(2~{R})-2-[5-[3-chloranyl-2-methyl-5-(4-methylpiperazin-1-yl)-4-oxidanyl-phenyl]-6-ethyl-thieno[2,3-d]pyrimidin-4-yl]oxy-3-phenyl-propanoic 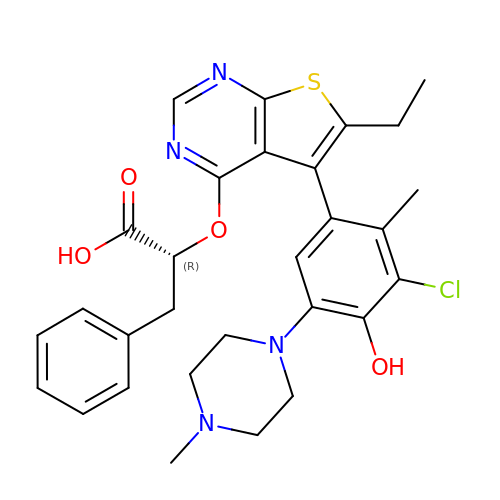acid | C29 H31 Cl N4 O4 S | OZKTZQZOQQOTJP-OAQYLSRUSA-N>[2x]GPLGSMSKSAVSPMMQQYLGIKAQHTDKLVFYRMGDFYELFLDDAVEAAKLLDITLTTRGQMDGVPIKMAGVPFHAAEQYLARLVKLGKSVAICEQVGEVGAGKGPVERKVVRIVTPGTLTDSALLEDKETNRIVAVSPDKKYIGLAWASLQSGEFKTKLTTADKLNDELARLQAAEILLPDSKNAPQLQTASGVTRLNAWQFAADAGEKLLTEYFGCQDLRGFGLDSKEHAVSIGAAGALLNYIRLTQNLMPQHLDG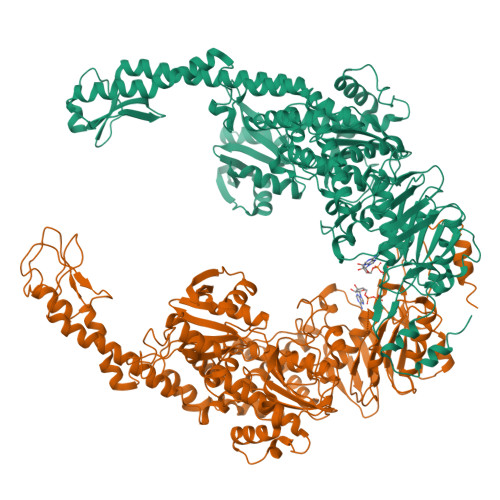LSLETDSQYIGMDAATRRNLEITQTLSGKKTPTLFSILDGCATHMGSRLLALWLHHPLRNRAHIRARQEAVTALESQYEPLQCHLKSIADIERIAARIAVGNARPRDLASLRDSLFELAQIDLSATGSSLLETLKAVFPETLPVAETLKAAVMPEPSVWLKDGNVINHGFHPELDELRRIQNHGDEFLLDLEAKERERTGLSTLKVEFNRVHGFYIELSKTQAEQAPADYQRRQTLKNAERFITPELKAFEDKVLTAQDQALALEKQLFDGVLKNLRTALPQLQKAAKAAAALDVLSTFSALAKERNFVRPEFADYPVVHIENGRHPVVEQQVRHFTANHTDLDHKHRLMLLTGPNMGGKSTYMRQVALIVLLAHTGCFVPADAATIGPVDQIFTRIGASDDLASNRSTFMVEMSETAYILHHATEQSIVLMDEVGRGTSTFDGLALAHAIAEHLLQKNKSFSLFATHYFELTYLPEAHAAAVNMHLSALEQGRDIVFLHQIQPGPAGKSYGIAVAKLAGLPVRALKAAQKHLNGLENQAAANRPQLDIFSTMPSEKGDEP>MARKHIYIAYTGGTIGMKKSDHGYVPVAGFMEKQLASMPEFHRPEMPLFTIHEYDPLMDSSDMTPADWQLIADDIAANYDKYDGFVILHGTDTMAYTASALSFMFENLGKPVIVTGSQIPLADLRSDGQANLLNALHVAANYPINEVTLFFNNRLMRGNRSRKSHADGFSAFSSPNLPPLLEAGINIELSTNVKVDEKPSGEFKVNPITPQPIGVITMYPGISHEVIRNTLLQPVNAMILLTFGVG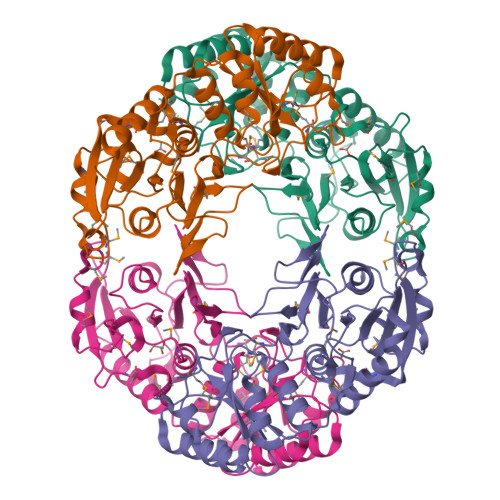NAPQNPELLAQLKAASERGVIVVNLTQCLAGKVNMGGYATGCALADAGVISGYDMTPEAALAKLHYLLSQNLSYEEVKAKMQQVLRGEMTL[4x]> SNKKQSNRLTEQHKLSQGVIGIFGDYAKAHDLAVGEVSKLVKKALSNEYPQLSFRYRDSIKKTEINEALKKIDPDLGGTLFVSNSSIKPDGGIVEVKDDYGEWRVVLVAEAKHQGKDIINIRNGLLVGKRGDQDLMAAGNAIERSHKNISEIANFMLSESHFPYVLFLEGSNFLTENISITRPDGRVVNLEYNSGILNRLDRLTAANYGMPINSNLCINKFVNHK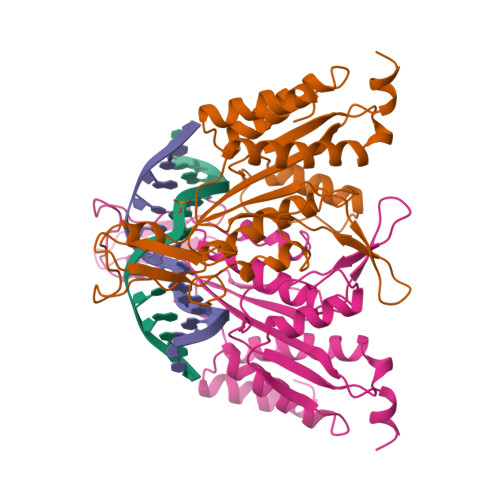DKSIMLQAASIYTQGDGREWDSKIMFEIMFDISTTSLRVLGRDLFEQLTSK> GPGYQSLDGLAKQKREELLQASVSPYHLFSDVADVTAFRSNLLSWYDQEKRDLPWRNLAKEEANSDRRAYAVWVSEVMLQQTQVATVIDYYTRWMQKWPKLQDLASASLEEVNQLWSGLGYYSRGRRLQEGARKVVEELGGHMPRTAETLQQLLPGVGRYTAGAIASIAFDQV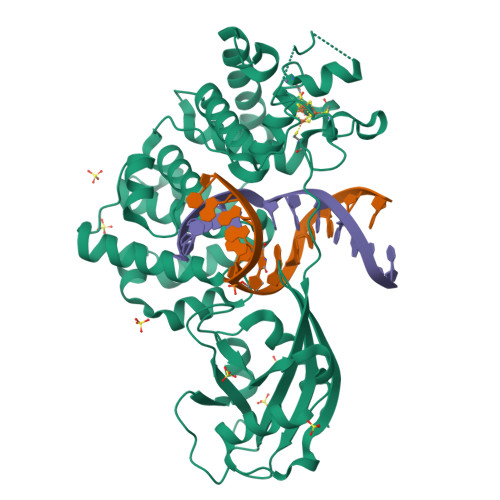TGVVDGNVLRVLCRVRAIGADPTSTLVSHHLWNLAQQLVDPARPGDFNQAAMELGATVCTPQRPLCSHCPVQSLCRAYQRVQRGQLSALPGRPDIEECALNTRQCQLCLTSSSPWDPSMGVANFPRKASRRPPREEYSATCVVEQPGAIGGPLVLLVQRPDSGLLAGLWEFPSVTLEPSEQHQHKALLQELQRWCGPLPAIRLQHLGEVIHIFSHIKLTYQVYSLALDQAPASTAPPGARWLTWEEFCNAAVSTAMKKVFRMYEDHRQGTRKGSKRSQVCPPSSR> SLLDVVVENNLDIDGFGACEGTL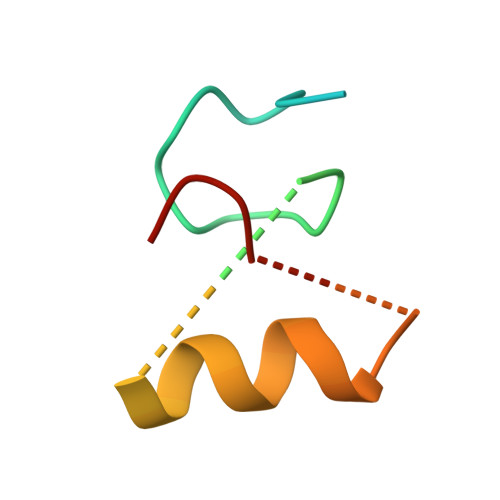ACSTCHLIFEDHIYEKLDAITDEENDMLDLAYGLTDRSRLGCQIC> MERNKLARQIIDTCLEMTRLGLNQGTAGNVSVRYQDGMLITPTGIPYEKLTESHIVFIDGNGKHEEGKLPQSEWRFHMAAYQSRPDANAVVHNHAVHCTAVSILNRSIPAIHYMIAAAGGNSIPCAPYATFGTRELSEHVALALKNRKATLLQHHGLIACEVNLEKALWLAHE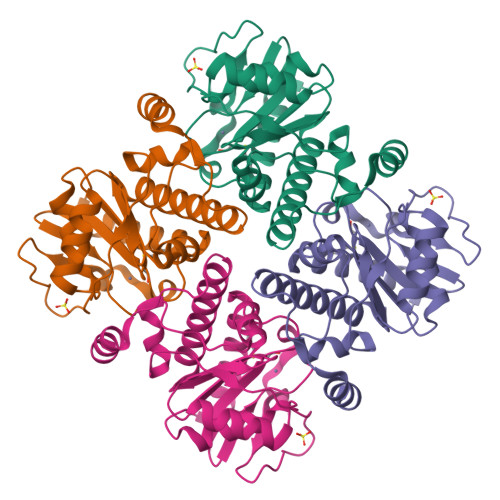VEVLAQLYLTTLAITDPVPVLSDEEIAVVLEKFKTFGLRIEE> MQWVKQLNVVFCTMLFSFSSYANLSDFKVA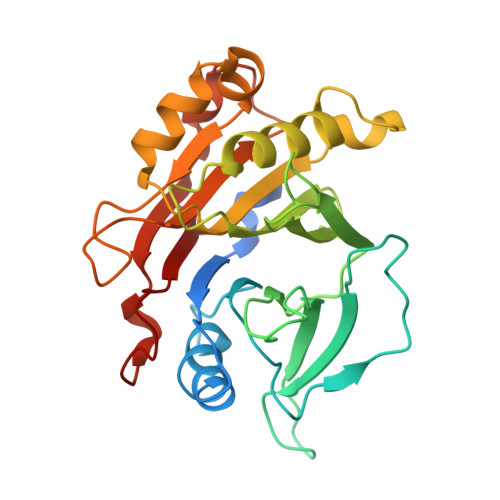TWNLQGSSAVNESKWNINVRQLLSGEQGADILMVQEAGSLPSSAVRTSRVIQHGGTPIEEYTWNLGTRSRPNMVYIYYSRLDVGANRVNLAIVSRRQADEAFIVHSDSSVLQSRPAVGIRIGTDVFFTVHALATGGSDAVSLIRNIFTTFTSSPSSPERRGYSWMVVGDFNRAPVNLEAALRQEPAVSENTIIIAPTEPTHRSGNILDYAILHDAHLPRREQARERIGASLMLNQLRSQITSDHFPVSFVHDR> AMRQCAIYGKGGIGKSTTTQNLVAALAEMGKKVMIVGCDPKADSTRLILHSKAQNTIMEMAAEAGTVEDLELEDVLKAGYGGVKCVESGGPEPGVGCAGRGVITAINFLEEEGAYEDDLDFVFYDVGDVVCGGFAMPIRENKAQEIYIVCSGEMMAMYAANNISKGIVKYANSGSVRLGGLICNSRNTDREDELIIALANKLGT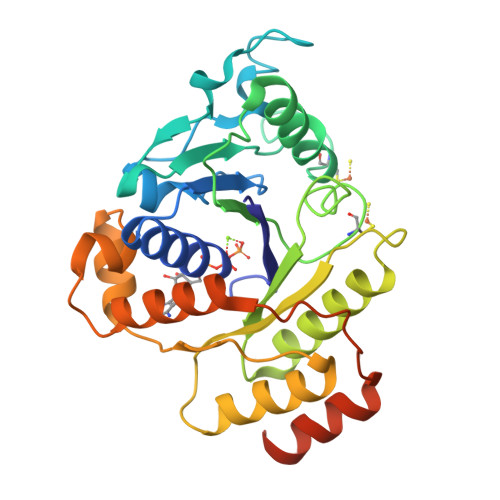QMIHFVPRDNVVQRAEIRRMTVIEYDPKAKQADEYRALARKVVDNKLLVIPNPITMDELEELLMEFGIMEVEDESIVGKTAEEV> NAMSVKIFN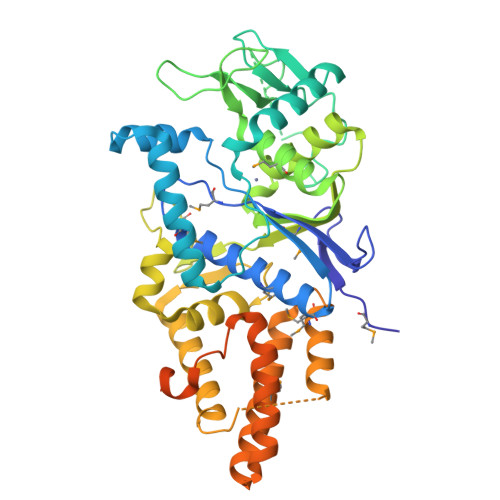SLTKQKEIFKPIESGKVKLYVCGMTVYDYMHIGHGRSWIIFDMVVRYLRMRGYEVTFVRNITDIDDKIIKRAGENKESPAALAERFIQILHEDEKALRVLSPDQEPRATQYVPEIIKLIQKLLDNQYAYTGQNGDVFFDVRRFKDYGKLSHRHLDELQAGARVEVSDSKRDPLDFVLWKKAKPGEPKWDSPWGEGRPGWHIECSAMSSSILGQPFDIHGGGLDLKFPHHENEIAQSEAGEEKPFVKLWMHAGLLEINKEKMSKSLGNIISIREALKESDVEVLRYFLLSGHYRNPLSYSKENLENGRLALERFYLALRGLPVVNHEKTSSYTDRFYEAMDDDFNTPIAFALLFEMVREINRFRDNNQIEKAAVLAAELKCLGNIFGLLQYSPEQFLQGAKKEADVQEIKKLIDQRNEARAKKDWKTADQIRDQLTDLGVAIEDSSDGTSWRQE> MRERPHTSGH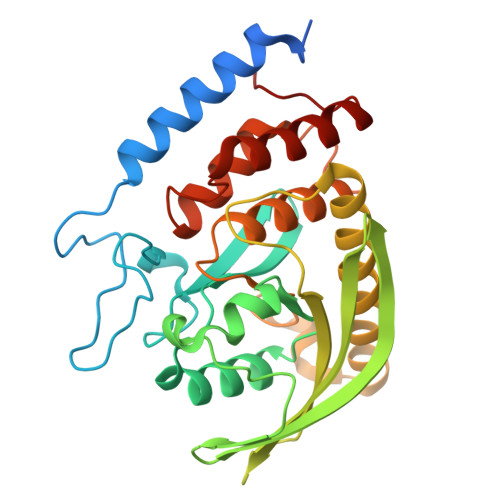HGAGEARATAPSTVSPYGPEARAELSSRLTTLRNTLAPATNDPRYLQACGGEKLNRFRDIQCRRQTAVRADLNANYIQVGNTRTIACQYPLQSQLESHFRMLAENRTPVLAVLASSSEIANQRFGMPDYFRQSGTYGSITVESKMTQQVGLGDGIMADMYTLTIREAGQKTISVPVVHVGNWPDQTAVSSEVTKALASLVDQTAETKRNMYESKGSSAVADDSKLRPVIHCRAGVGRTAQLIGAMCMNDSRNSQLSVEDMVSQMRVQRNGIMVQKDEQLDVLIKLAEGQGRPLLNS>[2x]SNATFVLKEFDALKSHFNDTVKIILQREKKDKIEDLPNPRKEELQFLTAVLNQLEAKIDELKPRSLASYVHVFYGAMLLVCKDVENNLRVMEKKENSLLFTRLMDGMGISDENIPTSEQNIMFYRGLNKFLNFIYESNDSRKGLKKEHFLQVLSLKKIYSLAKLSYEQEEAAENNALAKLTADGKTKANANSFHVEKPIDSSIVEQFKSWDEMKGALH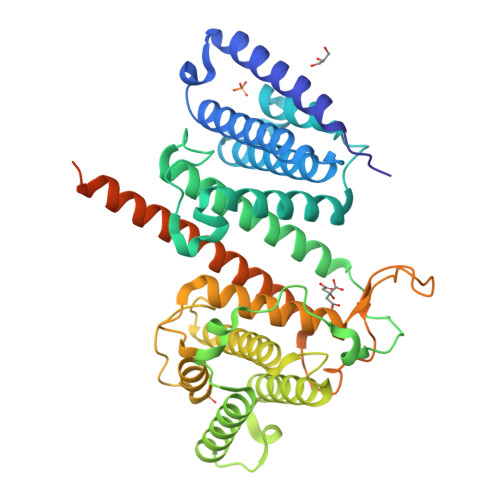QLILDELSDKNVAKISALSQARSAQLKFLQTMAEQLDKIPNQSLEPSEKMAILAGAMYIVRGQIAQEYGKDPLSNDKISATVIHTGLSTILHANADCCEDKEVLIAAANKFIRHMVIERPEQSNKKITKESVRENNMFSDIAGFQLISVLTLIQNMIKTCRTDAIEACVTKRKEELEALKPKKEGYSIASSVTGYVGSWFKKAPSMSEEDEEDDLKDQNTAEETSKPTV1-{6-[(3R)-3-methylmorpholin-4-yl]-2-(1H-pyrrolo[2,3-b]pyridin-4-yl)pyrimidin-4-yl}cyclopropane-1-sulfonamide | C19 H22 N6 O3 S | 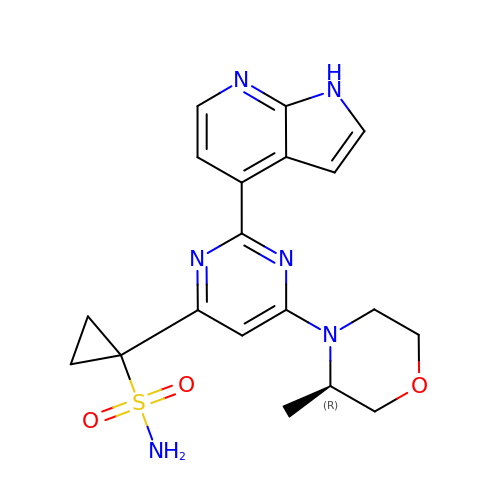XKCQCSLVYCUDFM-GFCCVEGCSA-N> YFQGHMMIHAPRRWVERHKQVQVLPQNAVEKLISMNELIELVIECGLCDKTSIKKMYDKINTYQFMWCIVDTIPASQYAEEIFKSSLHFLCALFLVDDAVESYSANEMQDLSRSYDILEKEVCKTFPNFPSINEMKESLMHLRNPFDRSSITFCMQYVNKITAILLEEGNTPHHVVYNLRRRTSNAISIAFQAVLIKSKCGSIITSHEMLWRRVFDGLVILFYQFGELISGATETAQQHITVVTELRMLGCLYCIVINDLYSYQRDKLASSDNMIKTWLLEKTVSSLSEATARCSQILDAIMKYMYQRVEQCMQSNPGCPQLESLLETTIYTTVGWIRSHTTVVPRYSESQLKVALVEVEERELPKWLAEKDEYGWNVVEKFVETLNDEKHKGILDALQGIADGRDQLLKTQ

To address these issues, we conducted genome mining of terpene synthases from the sea whip coral Paramuricea clavata, resulting in the discovery of a biflorane synthase PcTS1. To fill the research gaps of the mechanism and structure in marine biflorane biosynthesis, we performed genome mining and biochemical characterization of sea whip coral–derived TSs, leading to the discovery of one biflorane TS, PcTS1, using GGPP as the substrate. Isotopic labeling studies, together with calculations, elucidate a cascade of 1,10-cyclization, 1,3-hydride shift, 1,6-cyclization, 1,2-hydride shift, 2,6-cyclization, cyclopropane ring opening, and deprotonation by the generated pyrophosphate, forming the biflorane scaffold. Our work demonstrated the mechanism of marine biflorane formation, elucidated the second crystal structure of a coral terpene synthase, and realized the terpene skeleton expansion.

The structural basis of the cyclization mechanism was studied by determining the crystal structure of PcTS1. Followed by several failure crystallization efforts with full-length PcTS1, we expressed and purified a truncated form of PcTS1, PcTS1ΔN1–5, which lacks the first five N-terminal amino acids with catalytic activity unaffected. However, it distinguishes itself with the absence of one helix (K), the elongation of two helices (H and M), and the presence of an additional helix (O) because of an insertion. Notably, PcTS1 shares a remarkable structural resemblance with microbial TS-like proteins, in concert with the similarities observed in ErTC-2 (15). PcTS1 exhibits an overall structure that closely aligns with the tFold-generated model of PcTS1, with a root-mean-square deviation of 0.94 Å for the Cα atoms. However, the tFold-based model of PcTS1 features two additional helices (K and P) and helix M in the apo form of PcTS1 is split into two helices (M and M1), underscoring the significance of protein crystal structure analysis for achieving more precise outcomes. (D) Amino acid residues of the conservative region in apo-PcTS1, DDXXE motif on helix D, NSD/DTE motif on helix H, and RY motif on the loop region near helix J. In the QM/MM calculation, the A+ is observed to bind within a hydrophobic active pocket comprising aromatic residues (F64, F93, F221, W335, and H339), hydrophobic residues (I59, A189, G216, V218, I254, V343, and P344), and polar residues (C253 and S338). Notably, R212, D215, and S270 were identified as critical for activity.>MGEVALEGSNLEKMIQLFLQLDRNRDDIVDENELRQACAEHKLPEEEVSRWLDMFDADENGKITLEEFCRALGLRTAEMRVEKMEREEVRAGRGRPMPEDVEVIASTMSQEKKVEVTEKFKEFLAKTGGKPEDMNLVVKQLKDYLDERHGRVWQTLVLTGSYWMKFSHEPFMSL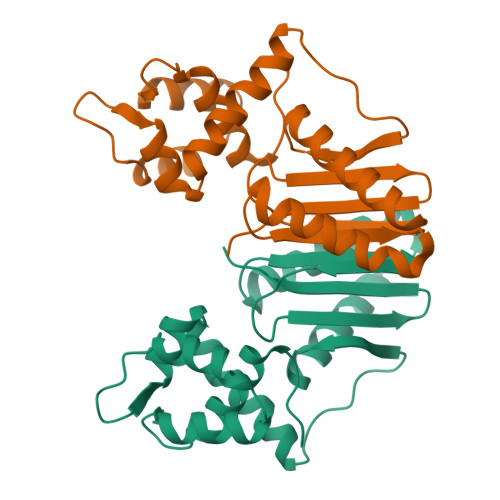QFKVGPNIVLVWRTPSN[2x]> MRGSHHHHHHGIPLPGRAMGTRDDEYDYLFKVVLIGDSGVGKSNLLSRFTRNEFNLESKSTIGVEFATRSIQVDGKTIKAQIWDTAGLERYRAITSAYYRGAVGALLVYDIAKHLTYENVERWLKELRDHADSNIVIMLVGNKSDLRHLRAVPTDEARAFAEKNGLSFIETSALDS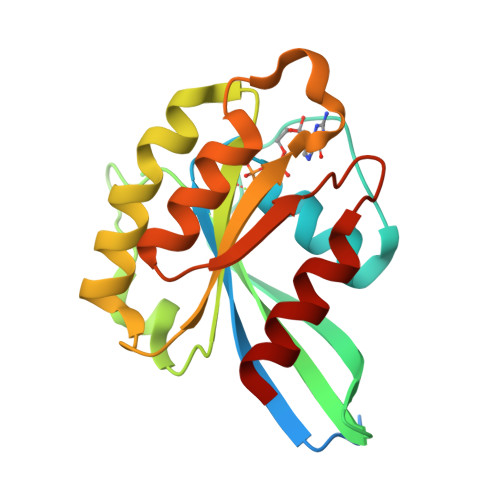TNVEAAFQTILTEIY> QVVVLGYGTGQKLSTVSGSVAKVSSEKLAEKPVANIMDALQGQVAGMQVMTTSGDPTAVASVEIHGTGSLGASSAPLYIVDGMQTSLDVVATMNPNDFESMSVLKDASATSIYGARAANGVVFIQTKKGKMSERGRITFNASYGISQILNTKPLDNMMTGDELLDFQVKAGFWGNNQTVQKVKDMILAG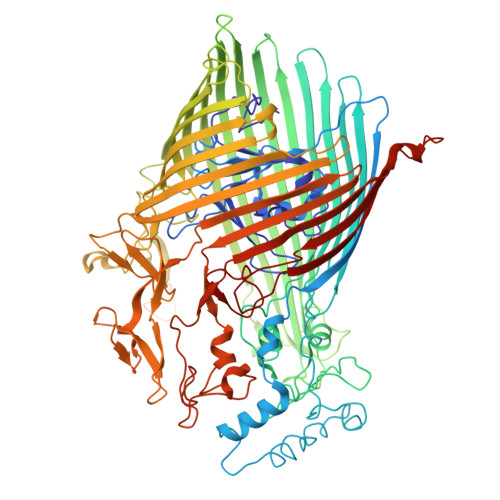AEDLYGNYDSLKDEYGKTLFPVDFNHDADWLKALFKTAPTSQGDISFSGGSQGTSYYASIGYFDQEGMAREPANFKRYSGRLNFESRINEWLKVGANLSGAIANRRSADYFGKYYMGSGTFGVLTMPRYYNPFDVNGDLADVYYMYGATRPSMTEPYFAKMRPFSSESHQANVNGFAQITPIKGLTLKAQAGVDITNTRTSSKRMPNNPYDSTPLGERRERAYRDVSKSFTNTAEYKFSIDEKHDLTALMGHEYIEYEGDVIGASSKGFESDKLMLLSQGKTGNSLSLPEHRVAEYAYLSFFSRFNYGFDKWMYIDFSVRNDQSSRFGSNNRSAWFYSVGGMFDIYNKFIQESNWLSDLRLKMSYGTTGNSEIGNYNHQALVTVNNYTEDAMGLSISTAGNPDLSWEKQSQFNFGLAAGAFNNRLSAEVDFYVRTTNDMLIDVPMPYISGFFSQYQNVGSMKNTGVDLSLKGTIYQNKDWNVYASANFNYNRQEITKLFFGLNKYMLPNTGTIWEIGYPNSFYMAEYAGIDKKTGKQLWYVPGQVDADGNKVTTSQYSADLETRIDKSVTPPITGGFSLGASWKGLSLDADFAYIVGKWMINNDRYFTENGGGLMQLNKDKMLLNAWTEDNKETDVPKLGQSPQFDTHLLENASFLRLKNLKLTYVLPNSLFAGQNVIGGARVYLMARNLLTVTKYKGFDPEAGGNVGKNQYPNSKQYVAGIQLSF>[2x]GLEVDNNSLLRNIYSTIVYEYSDIVIDFKTSHNLVTKKLDVRDARDFFINSEM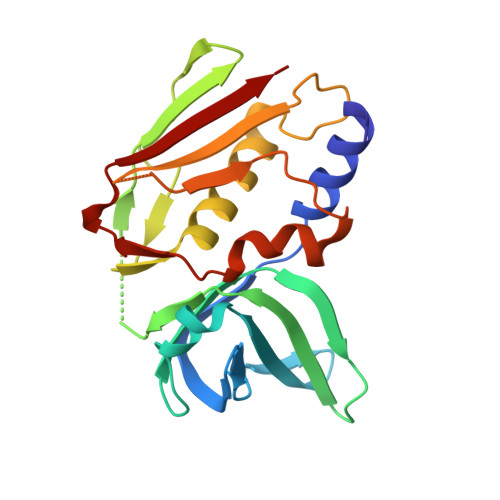DEYAANDFKTGDKIAVFSVPFDWNYLSKGKVTAYTYGGITPYQKTSIPKNIPVNLWINGKQISVPYNEISTNKTTVTAQEIDLKVRKFLIAQHQLYSSGSSYKSGRLVFHTNDNSDKYSFDLFYVGYRDKESIFKVYKDNKSFNIDKIGHLDIEIDS>MEKMDNLEVKAKINQGLYKITPRHKGTSFIWNVLADIQKEDDTLVEGWVFCRKCEKVLKYTTRQTSNLCRHKCCASLKQSRELKTVSADCKKEAIEKCAQWVVRDCRPFSAVSGSGFIDMIKFFIKVGAEYGEHVNVEELLPSPITLSRKVTSDAKEKKALISREIKSAVEKDGASATIDLWTDNYIKRNFLGVTLHYHENNELRDLILGLKSLDFERSTAENIYKKLKAIFSQFNVEDLSSIKFVTDRGANVVKSLANNIRINCSSHLLSNVLENSFEETPELNMPILACKNIVKYFKKANLQHRLRSSLKSECPTRWNSTYTMLRSILDNWESVIQILSEAGETQRIVHINKSIIQTMVNILDGFERIFKELQTCSSPSLCFVVPSILKVKEICSPDVGDVADIAKLKVNIIKNVRIIWEENLSIWHYTAFFFYPPALHMQQEKVAQIKEFCLSKMEDLELINRMSSFNELSATQLNQSDSNSHNSIDLTSHSKDISTTSFFFPQLTQNNSREPPVCPSDEFEFYRKEIVILSEDFKVMEWWNLNSKKYPKLSKLALSLLSIPASSAASERTFSLAGNIITEKRNRIGQQTVDSLLFLNSFYKNFCKLDI[6x]

The Hermes DNA transposon is a member of the eukaryotic hAT superfamily, and its transposase forms a ring-shaped tetramer of dimers. The Hermes transposase is composed of 612 amino acids and is organized in four domains. Architecturally, the Hermes transposase is unusual as it spontaneously forms a ring-shaped tetramer of dimers. All hAT transposases are predicted to contain an N-terminal BED zinc-finger domain organized around a conserved CCHH or CCHC motif that coordinates Zn2+13, but no structural information is available for Hermes as the constructs used in previous structural work lacked the first 78 amino acids.

On the basis of the SEC and MP experiments, for cryo-EM studies we selected the 8 + LE-TIR + 30 oligonucleotide as it contained both flanking region and the longest transposon DNA. In order to resolve the interactions between the BED domains and DNA, we performed multi-body 3D refinement on the three best 3D classes (regardless of the oligomerization state of the transposase) using masks to divide the transpososome into three bodies. There are also two DNA-bound BED domains (in green) that have been contributed by the B dimer. Thus, three BED domains bind to each DNA. The two LE-DNAs are antiparallel, with each TIR interacting with a different Hermes dimer next to the 3’-end of the other oligonucleotide. The 8 + TIR-LE + 30 DNA includes the TIR and STR1 through STR4. STR1 is clearly bound by the BED domain that belongs to the same Hermes protomer (A1 or C1) that also binds to the TIR as indicated by distinct linker density between the BED domain and the dimerization domain (DD in Fig. 1c). Furthermore, the STR2 motifs are also bound in the hexameric Hermes transpososome where only one equatorial dimer is present at the position of dimer B. Therefore, we conclude that the equatorial Hermes dimer B engages both its BED domains with the STR2 motifs. STR4 was not bound by any BED domain; rather, the 3’-end of each oligonucleotide (bp 36–47) was positioned similarly as the TIR entering the catalytic domain of the A2 or C2 protomer, with bp 47 sitting at the place of the TIR bp 3. In the LE-LE complex, although the two ends were antiparallel (an arrangement that clearly cannot support transposition), each of the first three STRs within the first 35 bp of the LE interacted with a BED domain originating from three different Hermes dimers (left).1-[1-(3-fluorophenyl)-6,7-dihydro-4~{H}-pyrazolo[4,3-c]pyridin-5-yl]propan-1-one | C15 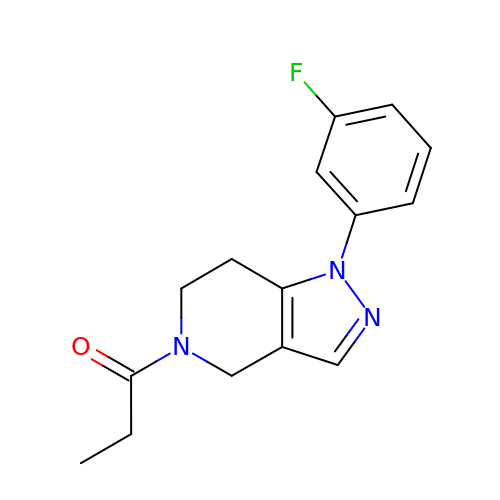H16 F N3 O | PBPQRCMCEYVHIP-UHFFFAOYSA-N>[2x]MAHHHHHHMSMRLIWAQSTSGIIGRDNSIPWRLPEDLARFKEMTMGHPVVMGRLTWESLPASVRPLPGRRNIVVTRDADYRAEGAEVVTDLP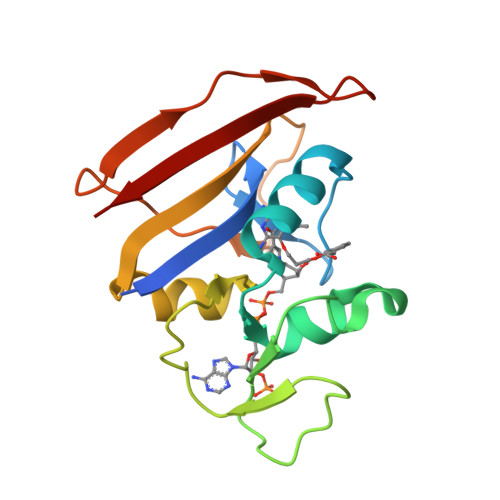DEPDAWVIGGAQIYAMALARADRCEVTEVDIALTPLDGDARAPVLDDSWVATTGEWQTSTSGLRFRFCSYRR> DGNAGLLAEPQIAMFCGRLNMHMNVQNGKWDSDPSGTKTCIDTKEGILQYCQEVYPELQITNVVEANQPVTIQNWCKRGRKQCKTHPHFVIPYRCLVGEFV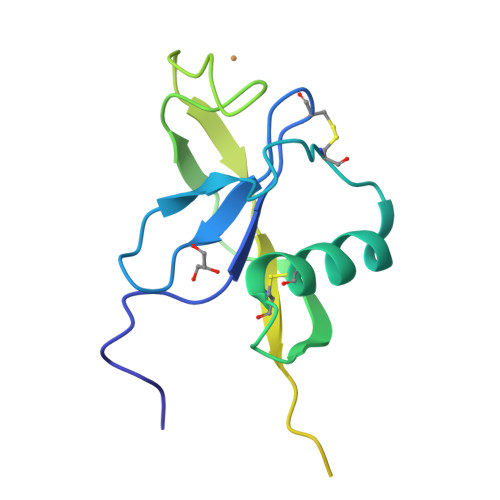SDALLVPDKCKFLHQERMDVCETHLHWHTVAKETCSEKSTNLHDYGMLLPCGIDKFRGVEFV>[4x]GA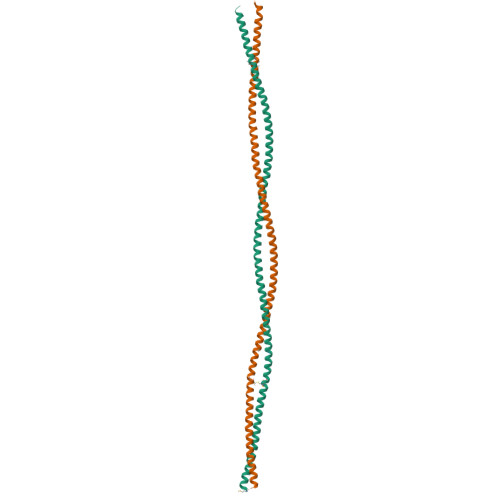MESTVNALTSELRDLRAQREEAAAAHAQEVRRLQEQARDLGKQRDSCMREAEELRTQLRLMEDARDGLRRELLEAQRKLRESQEGREVQRQEAGELRRSLGEGAKEREALRRSNEELRSAVKKAESERISLKLANEDKEQKLALLEEARTAVGKEAGELRTGLQEVERSRLEARRELQELRRQMKMLDSENTRLGRELAELQGRLALGERAEW>[2x]GAMGSYDWLPRLSKENFNAAPVTCFPHAPGCEVWDNLGVGMKVEVENTDCDSIEVIQPGQTPTSFWVATILEIKGYKALMSYEGFDTDSHDFWVNLCNAEVHSVGWCATRGKPLIPPRTIEHKYKDWKDFLVGRLSGARTLPSNFYNKINDSLQSRFRLGLNLECVDKDRISQV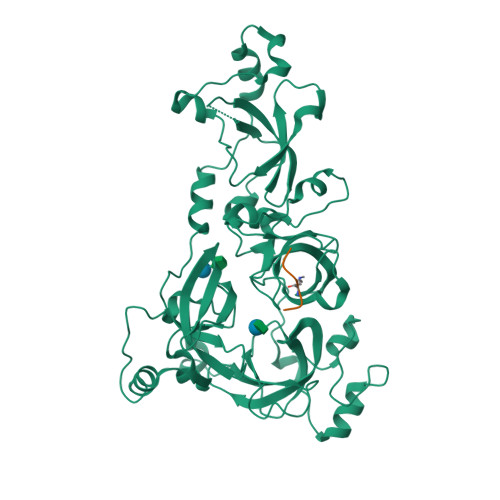RLATVTKIVGDRLFLRYFDSDDGFWCHEDSPIIHPVGWATTVGHNLAAPQDYLERMLAGREAMIEVHEDDATIELFKMNFTFDEYYSDGKTNSFVEGMKLEAVDPLNLSSICPATVMAVLKFGYMMIRIDSYQPDASGSDWFCYHEKSPCIFPAGFCSVNNISVTPPNGYDSRTFTWEGYLSDTGAVAAGQHLFHDIIPDHGFEVGMSLECADLMDPRLVCVATVARVVGRLLKVHFDGWTDEYDQWLDCESADIYPVGWCVLVNHKLEGPPR;>HRKVLR[2x]> ANDPFTIVHGNTGKCIKPVYGWIVADDCDETEDKLWKWVSQHRLFHLHSQKCLGLDITKSVNELRMFSCDSSAMLWWKCEHHSLYGAARYRLALKDGHGTAISNASDVWKKGGSEESLCDQPYHEIYTRDGNSYGRPCEFPFLIDGTWHHDCILDEDHSGPWCATTLNYEYDRKWGICLKPENGCEDNWEKNEQFGSCYQFNTQTALSWKEAYVSCQNQGADLLSINSAAELTYLKEKEGIAKIFWIGLNQLYSARGWEWSDHKPLNFLNWDPDRPSAPTIGGSSCARMDAESGLWQSFSCEAQLPYVCRKPLNNTVELTDVWTYSDTRCDAGWLPNNGFCYLLVNESNSWDKAHAKCKAFSSDLISIHSLADVEVVVTKLHNEDIKEEVWIGLKNINIPTLFQWSDGTEVTLTYWDENEPNVPYNKTPNCVSYLGELGQWKVQSCEEKLKYVCKRKGEKLNDASSDKMCPPDEGWKRHGETCYKIYEDEVPFGTNCNLTITSRFEQEYLNDLMKKYDKSLRKYFWTGLRDVDSCGEYNWATVGGRRRAVTFSNWNFLEPASPGGCVAMSTGKSVGKWEVKDCRSFKALSICKKMS

pmcDEC205 (CD205 or Ly75) is an endocytic receptor highly expressed on the dendritic cells with antigen-presenting function and has been widely used as a receptor target in immune therapies. DEC205 belongs to the mannose receptor family, which also includes mannose receptor (MR), PLA2R, Endo180 (8), and FcRY. MR family members are type I transmembrane proteins with a large extracellular portion, a transmembrane helix, and a short cytoplasmic region. Their ectodomains contain an N-terminal cysteine-rich domain (CysR), a fibronectin type II domain (FnII), and eight (ten for DEC205) C-type lectin-like domains (CTLDs). The functional studies of DEC205 show that it can act as a receptor for dead cells and may recognize dead cells through cellular keratins in a pH-dependent manner, as acidification usually occurs during the event of apoptosis, but the mechanism of the interaction between DEC205 and keratins remains unclear.

To investigate the structure of the CysR∼CTLD3 (residues M1- S627) fragment, we expressed the fragment in insect cells and the purified protein was applied for crystallization screening. Crystals were obtained in 0.2 M Sodium Citrate with 20% PEG3350 around neutral pH (pH 6.5–7.4). X-ray diffraction data were collected and showed two crystal forms, one in space group C2 and the other in space group P1. The structures of the CysR∼CTLD3 fragment show a C-shaped conformation in both crystal forms and they are quite similar with the r.m.s. deviation of Cα atoms of 0.89 Å. The CysR∼CTLD2 region of DEC205 has an L-shaped conformation that is also found in the crystal structures of MR and Endo180 and the C-shaped conformation of the CysR∼CTLD3 fragment of DEC205 is similar to that of MR at acidic condition. The structure of the CysR domain of DEC205 has a trefoil shape, similar to the CysR domains of MR and Endo180. The structure of the FnII domain of DEC205 is also similar to that of MR and Endo180, consisting of two β-sheets and two conserved disulfide bonds. The structures of CTLD1 and CTLD2 of DEC205 exhibit typical CTLD fold, and the two domains are associated with each other with a hydrophobic interface as well as hydrogen bonds, suggesting that they might be tightly associated with each other, which is similar to MR and Endo180 (15, 39). Notably, the structure of the CLTD3 of DEC205 is different from the conventional CTLD fold with two unique loop regions (loop 1 and loop 2). Loop 1 (residue E521-C528) replaces a conserved α-helix in the conventional CTLDs, and loop 2 (residue T573-A592) becomes much longer and partially missing in the crystal structure.> RPEFDWQDPLVLEEQLTTDEILIRDTFRTYCQERLMPRILLANRNEVFHREIISEMGELGVLGPTIKGYGCAGVSSVAYGLLARELERVDSGYRSAMSVQSSLVMHPIYAYGSEEQRQKYLPQLAKGELLGCFGLTEPNSGSDPSSMETRAHYNSSNKSYTLNGTKTWITNSPMADLFVVWARCEDGCIRGFLLEKGMRGLSAPRIQGKF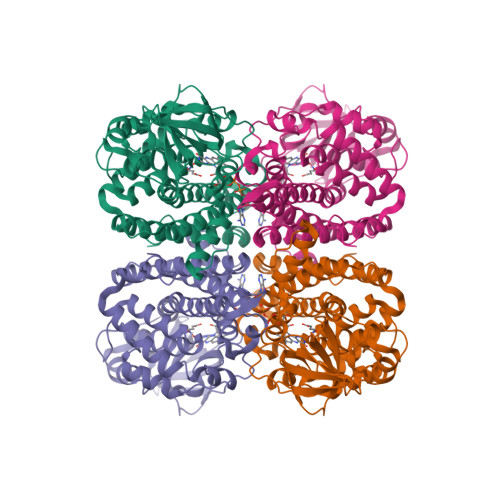SLRASATGMIIMDGVEVPEENVLPGASSLGGPFGCLNNARYGIAWGVLGASEFCLHTARQYALDRMQFGVPLARNQLIQKKLADMLTEITLGLHACLQLGRLKDQDKAAPEMVSLLKRNNCGKALDIARQARDMLGGNGISDEYHVIRHAMNLEAVNTYDGTHDIHALILGRAITGIQAFTASK>MEKNGNNRKLRVCVATCNRADYSKLAPIMFGIKTEPEFFELDVVVLGSHLIDDYGNTYRMIEQDDFDINTRLHTIVRGEDEAAMVESVGLALVKLPDVLNRLKPDIMIVHGDRFDALALATSAALMNIRILHIEGGEVSGTIDDSIRHAITKLAHYHVCCTRSAEQHLISMCEDHDRILLAGCPSYDKLLSAKNKDYMSIIRMWLGDDVKSKDYIVALQHPVTTDIKHSIKMFELTLDALISFNKRTLVLFPNIDAGSKEMVRVMRKKGIEHHPNFRAVKHVPFDQFIQLVAHAGCMIGNSSCGVREVGAFGTPVINLGTRQIGRETGENVLHVRDADTQDKILQALHLQFGKQYPCSKIYGDGNAVPRILKFLKSIDLQEPLQKKFCFPPVKENISQDIDHILEHHHHHH[4x]

Sialic acid biosynthesis in mammals starts by converting UDP-GluNAc into UDP and ManNAc, followed by phosphorylation of ManNAc at the sixth position. Catalysis of both reactions is carried out by the bifunctional enzyme GNE, which in human is composed of ~720 amino acid residues and divided into the epimerase part (~400 aa) and the kinase part (~300 aa). Being a key enzyme that catalyzes the rate-limiting step of sialic acid biosynthesis, GNE plays an important role in regulation of cell-surface sialyation level by binding to the downstream product CMP-Neu5Ac. To understand the mechanism by which CMP-Neu5Ac inhibits GNE, and to find out the difference between non-hydrolyzing and hydrolyzing UDP-GlcNAc epimerase, we crystallized the epimerase part of human GNE and determined its structure in the presence of substrate and inhibitor.

The crystal structure of the epimerase part of human GNE was determined at 2.7-Å resolution by single-wavelength anomalous diffraction (SAD) method using Se-Met enriched protein. Each asymmetric unit comprises four monomers (denoted A, B, C and D) in two homodimers. In addition, each dimer further forms a tetramer with a crystallographic dyad-related dimer, burying 1280 Å2 surface area on each monomer and showing the 222 point-group symmetry as observed in hemoglobin. Further away from the tetramer center, two pairs of CMP-Neu5Ac molecules intercalate between the dimers, burying an additional 390 Å2 surface area on each monomer. Only UDP was observed in the active site of each monomer despite the use of UDP-GlcNAc in crystallization. In fact, a ManNAc molecule was bound to a surface pocket formed by helices α1, α2 and α11 of monomer C. The pyrophosphate forms salt bridges to Arg19, Arg113 and Arg321. The allosteric inhibitor CMP-Neu5Ac is bound in an L-shaped conformation, forming an internal hydrogen bond between the CMP phosphate and the 8-OH of Neu5Ac. The carboxyl group of Neu5Ac, a characteristics of this negatively charged nine-carbon sugar, interacts with the three positively charged side chains of Arg263*, Arg266* and Lys267*. Therefore, at high CMP-Neu5Ac concentrations, the GNE tetramer assumes the closed, inactive, conformation to maintain the favored interactions with the inhibitor.The YfiBNR system contains three protein members and modulates intracellular c-di-GMP levels in response to signals received in the periplasm. YfiN is repressed by specific interaction between its periplasmic PAS domain and the periplasmic protein YfiR. YfiB is an OmpA/Pal-like outer-membrane lipoprotein that can activate YfiN by sequestering YfiR in an unknown manner. Previous studies suggested that in response to cell stress, YfiB in the outer membrane sequesters the periplasmic protein YfiR, releasing its inhibition of YfiN on the inner membrane and thus inducing the diguanylate cyclase activity of YfiN to allow c-di-GMP production.

We obtained two crystal forms of YfiB (residues 34–168, lacking the signal peptide from residues 1–26 and periplasmic residues 27–33), crystal forms I and II, belonging to space groups P21 and P41, respectively. The crystal structure of YfiB monomer consists of a five-stranded β-sheet (β1-2-5-3-4) flanked by five α-helices (α1–5) on one side. Each crystal form contains three different dimeric types of YfiB, two of which are present in both, suggesting that the rest of the dimeric types may result from crystal packing. Here, we refer to the two dimeric types as “head to head” and “back to back” according to the interacting mode, with the total buried surface areas being 316.8 Å2 and 554.3 Å2, respectively. The “head to head” dimer exhibits a clamp shape. The dimerization occurs mainly via hydrophobic interactions formed by A37 and I40 on the α1 helices, L50 on the β1 strands, and W55 on the β2 strands of both molecules, making a hydrophobic interacting core. The “back to back” dimer presents a Y shape. The dimeric interaction is mainly hydrophilic, occurring among the main-chain and side-chain atoms of N68, L69, D70 and R71 on the α2-α3 loops and R116 and S120 on the α4 helices of both molecules, resulting in a complex hydrogen bond network. The apo YfiB structure constructed beginning at residue 34 has a compact conformation of approximately 45 Å in length. Thus, YfiB alone represents an inactive form that may only partially insert into the PG matrix.

>GLSAEQIAVLQEQGFELRDEGWEFGMSSKVLFGNNLDRLNPDSRNTLTKIARALLAVDIDKVRLEGHTDNYGDEGYNQKLSERRAESVAAVFREAGMPAANIEVRGLGMSKPVADNKTRAGRSENRRVAIIVPAE[4x]> MGSHHHHHHSQDPMAYSTREILLALCIRDSRVHGNGTLHPVLEL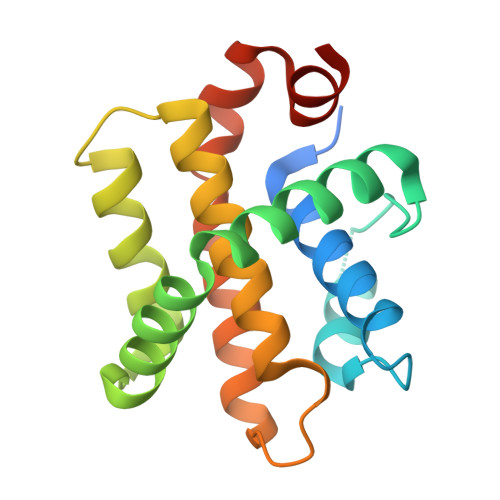AARETPLRLSPEDTVVLRYHVLLEEIIERNSETFTETWNRFITHTEHVDLDFNSVFLEIFHRGDPSLGRALAWMAWCMHACRTLCCNQSTPYYVVDLSVRGMLEASEGLDGWIHQQGGWSTLIEDNIPG2-{4-[(4-amino-2-methylpyrimidin-5-yl)methyl]-3-methylthiophen-2-yl}ethanol | C13 H17 N3 O S | 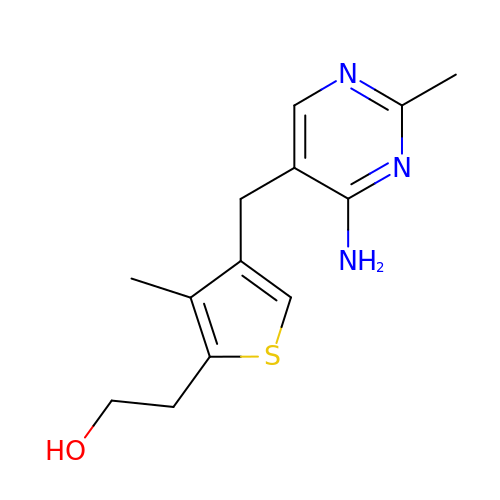HLBXMICRXICHJQ-UHFFFAOYSA-N> MNLKDSIGLRIKTERERQQMSREVLCLDGAELTVRQLIRIEKGESLPSLDRLSYIAKRLGKSMTELLDQDNITIPDEYYEMKNRLIKFPTYRNPDRIKSKLTLIEEVYEKFFDILPEEELLTLDILENILSFTSWEESPKVEEIYEDLFEQVKRKRKFSTNDLLVIDYYFFHLYGRKQYDKKLFERIIKRVLNQEIWTDDVYNIVLFNDLM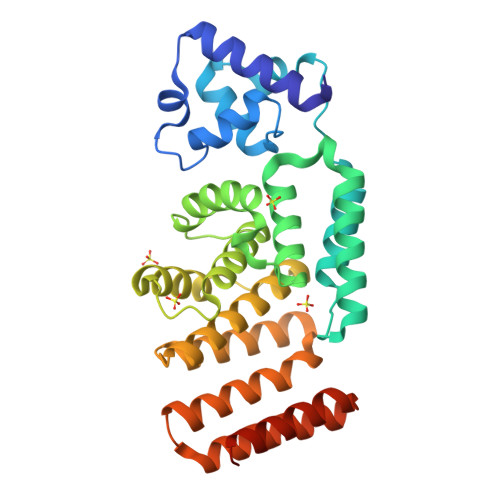AIAALKIFHNSFSDFLTVVDKALAVIEKSQLYSYKPSVFVLKAKYELLHKENKKEAAENYDKAIVFASVLEDSVLEESIKAGKLADGLGAGWSHPQFEK> AHMASDNYFRIHVKKLPEENKDAQGLWTWDDVEKPSENWPNGALSFKDAKKDDYGYYLDVKLKGEQAKKISFLINNTAGKNLTGDKSVEKLVPKMNEAWLDQDYKVFSYEPQPAGTVRVNYYRTDGNYDKKSLWYWGDVKNPSSAQWPDGTDFTATGKYGRYIDIPLNEAAREFGFLLLDESKQGDDVKIRKENYKFTDLKNHSQIFLKDDDESIYTNPYYVHDIRMTGAQHVGTSSIESSFSTLVGAKKEDILKHSNITNHLGNKVTITDVAIDEAGKKVTYSGDFSDTKHPYTVSYNSDQFTTKTSWRLKDETYSYDGKLGADLKEEGKQVDLTLWSPSADKVSVVVYDKNDPDKVVGTVALEKGERGTWKQTLDSTNKLGITDFTGYYYQYQIERQGKTVLALDPYAKSLAAWNSDDSKIDDAHKVAKAAFVDPAKLGPQDLTYGKIHNFKTREDAVIYEAHVRDFTSDPAIAKDLTKPFGTFEAFIEKLDYLKDLGVTHIQLLPVLSYYFVNELKNHERLSDYASSNSNYNWGYDPQNYFSLTGMYSSDPKNPEKRIAEFKNLINEIHKRGMGAILDVVYNHTAKVDLFEDLEPNYYHFMDADGTPRTSFGGGRLGTTHHMTKRLLIDSIKYLVDTYKVDGFRFDMMGDHDAASIEEAYKAARALNPNLIMLGEGWRTYAGDENMP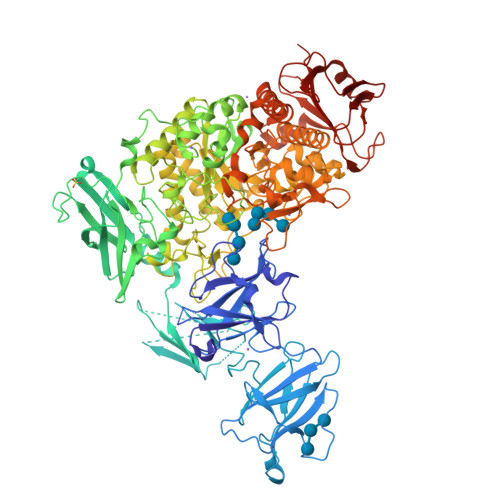TKAADQDWMKHTDTVAVFSDDIRNNLKSGYPNEGQPAFITGGKRDVNTIFKNLIAQPTNFEADSPGDVIQYIAAHDNLTLFDIIAQSIKKDPSKAENYAEIHRRLRLGNLMVLTAQGTPFIHSGQEYGRTKQFRNPAYRTPVAEDKVPNKSHLLRDKDGNPFDYPYFIHDSYDSSDAVNKFDWTKATDGKAYPENVKSRDYMKGLIALRQSTDAFRLKSLQDIKDRVHLITVPGQNGVEKEDVVIGYQITAPNGDIYAVFVNADEKAREFNLGTAFAHLRNAEVLADENQAGPVGIANPKGLEWTEKGLKLNALTATVLRVSQN> MTTVPDLESDSFHVDWYRTYAELRETAPVTPVRFLGQDAWLVTGYDEAKAALSDLRLSSDPKKKYPGVEVEFPAYLGFPEDVRNYFATNMGTSDPPTHTRLRKLVSQEFTVRRVEAMRPRVEQITAELLDEVGDSGVVDIVDRFAHPLPIKVICELLGVDEKYRGEFGRWSSEILVMDPERAEQRGQAAREVVNFILDLVERRRTEPGDDLLSALIRVQDDDDGRLSADELTSIALVLLLAGFETSVSLIGIGTYLLLTHPDQLALVRRDPSALPNAVEEILR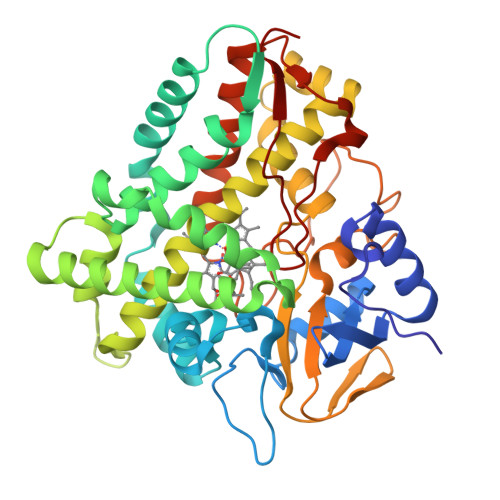YIAPPETTTRFAAEEVEIGGVAIPQYSTVLVANGAANRDPKQFPDPHRFDVTRDTRGHLSFGQGIHFCMGRPLAKLEGEVALRALFGRFPALSLGIDADDVVWRRSLLLRGIDHLPVRLDG> AEAGITGTWYNQLGSTFIVTAGADGALTGT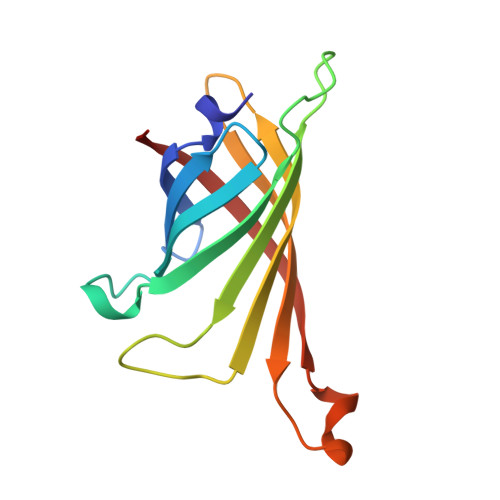YESAVGNAESRYVLTGRYDSAPATDGSGTALGWTVAWKNNYRNAHSATTWSGQYVGGAEARINTQWLLTSGTTEANAWKSTLVGHDTFTKVKP> MAHHHHHHVGTMKRKTGFFFDERCFWHSTGLHAVTLPVGGWVQPPAGGGHAESPETKRRMKNLMDVSGLTPQLALRSAAPASLEDLRRIHPDSYLERFKAISDNGGGMLGKEAPLGPGSYEIACLSAGLACAAVEAVLKGELDNAYSLSRPPGHACLPDQSMGFCFLANIPIAVERAKAQLGLGKVAIIDWDVHHGNGTQHIYLQRDDVLTISLHQDGCFPPGYAGEDDRGVGAGEGYNINIPLLAGAGDDSWRYALETIVIPALARFEPELIIIACGYDANAMDPLARMQLHSDSFRAMTEQVQQAADRLCGGKLVMVHEGGYAESYVPFCGLAVMEALSGIRTEVQDPLLEFIQQQQPRATFAQFQRQAIDRLAQQFGLQ

Classical Zn2+-dependent deac(et)ylases play fundamental regulatory roles in life and are well characterized in eukaryotes regarding their structures, substrates and physiological roles. Structurally, these enzymes are composed of a central eight-stranded parallel β-sheet flanked by α-helices on each site, known as the α/β-arginase/deacetylase fold. All active site residues were conserved, as shown by the multiple sequence alignment and the structural alignment, suggesting a general acid/base catalytic mechanism for the bacterial enzymes as described for the eukaryotic counterparts. These enzymes mediate catalysis using a penta-coordinated catalytic Zn2+ ion coordinated by two aspartates and a histidine (KpHdaH (1b): Asp181, Asp269, His183).

A double-His motif, (KpHdaH (1b): His143/His144) plays an important role during catalysis. The first His (KpHdaH: His143) of this tandem His motif acts as an electrostatic catalyst during catalysis, i.e. it orients and polarizes the catalytic water molecule, and it is itself oriented and polarized by an Asp (KpHdaH (1b): Asp179). The second His (KpHdaH: His144) acts as a general base abstracting a proton from the catalytic water molecule, thereby activating the water molecule for nucleophilic attack on the carbonyl carbon of the acetyl/amide-group, i.e. the acetyl-lysine, the acetylated polyamine or the small molecule amide. A mutation of the second His in KpHdaH (KpHdaH H144A) leads to an inactivation of the enzyme while not affecting the overall conformation. We also analyzed catalytically inactive enzymes obtained by mutation of an active site catalytic His residue, as control.>[2x]MAHHHHHHVDDDDKMSLLDAHIPQLIASHTAFAA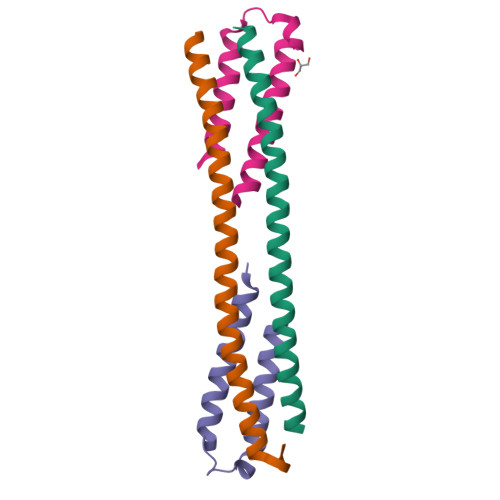KAGLMRHTIGQAEQQAMSAQAFHQGESAAAFQGAHARFVAAAAKVNTLLDIAQANLGEAAGTYVAADAAAASSYTGF;>MSQIMYNYPAMMAHAGDMAGYAGTLQSLGADIASEQAVLSSAWQGDTGITYQGWQTQWNQALEDLVRAYQSMSGTHESNTMAMLARDGAEAAKWGG[2x]>[2x]MKLSRSEFIKLGILTAAGISGLPGIKLSAQGTSSRKTVIVMGGGISGLYASYLLSKTGIKVQLIEATDRLGGRIRTVTDVSGNFLDLGAEWIQAEHRTAKSLIRELGLKTTDFEVQSDLFFGSYRKFGTWDISPKSQEILNKLVQMNSKINSTQQQELDRISFYNFLNYQGMSLEDLNILNF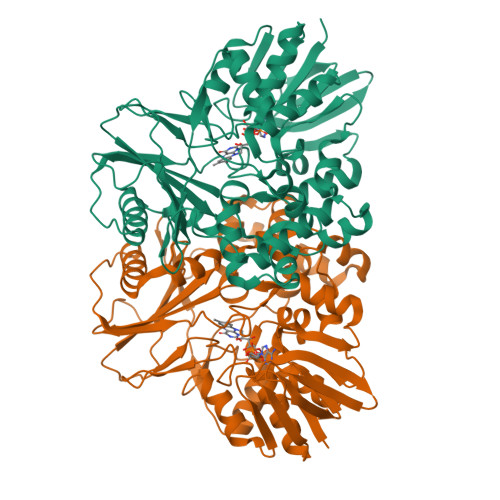KYSLYYGDSLRSLSAQKVLSDLVNFPKYNTRVEGGMETLTRALVSSLENTEIIFSDPVVSVSQGEGKVIVTTVSGKKIEGNACISTLPANQLTTIQWDPELDKEKKLSALRIRYSRIYKTFLMLREAPWTRGSFSAYSDSVAGFIYDAGTKINSEDKILGMISTGDRYDILASSTDAMKVEYIRLALESLGQGRELQVLRIQSSETSQSKFIPTGIATFPPGSYGSIISLLKPMDRIFFAGEHTAELNGTVEGALASAIRAVNQV7-oxo-5-phenyl-6-(propan-2-yl)-4,7-dihydropyrazolo[1,5-a]pyrimidine-3-carbonitrile | C16 H14 N4 O 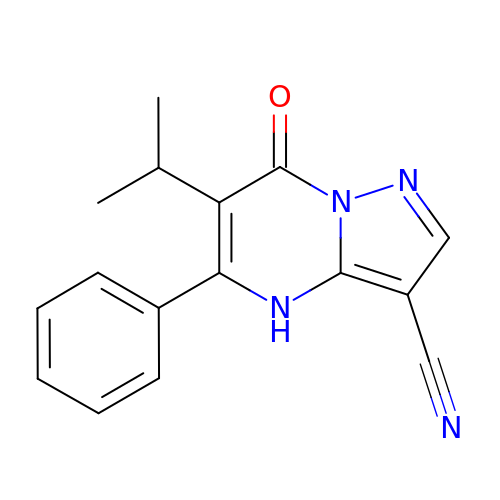| DHXKRMSKXLDZGY-UHFFFAOYSA-N>[2x]MSQQGLERRLLAGLQGLGLTINQAQRAVKHFGADALDRLEKDLFTLTEVEGIGFLTADKLWQARGGALDDPRRLTAAAVYALQLAGTQAGHSFLPRSRAEKGVVHYTRVTPGQARLAVETAVELGRLSEDDSPLFAAEAAATGEGRIYLPHVLRAEKKLASLIRTLLATPPADGAGNDDWAVPKKARKGLSEEQASVLDQLAGHRLVVLTGG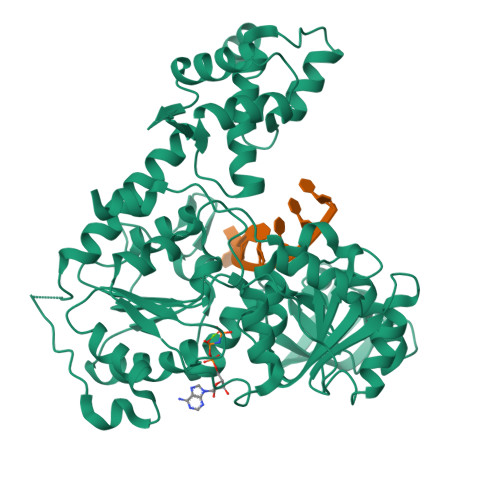PGTGKSTTTKAVADLAESLGLEVGLCAPTGKAARRLGEVTGRTASTVHRLLGYGPQGFRHNHLEPAPYDLLIVDEVSMMGDALMLSLLAAVPPGARVLLVGDTDQLPPVDAGLPLLALAQAAPTIKLTQVYRQAAKNPIIQAAHGLLHGEAPAWGDKRLNLTEIEPDGGARRVALMVRELGGPGAVQVLTPMRKGPLGMDHLNYHLQALFNPGEGGVRIAEGEARPGDTVVQTKNDYNNEIFNGTLGMVLKAEGARLTVDFDGNVVELTGAELFNLQLGYALTVHRAQGSEWGTVLGVLHEAHMPMLSRNLVYTALTRARDRFFSAGSASAWQIAAARQREARNTALLERIRAHLEHHHHHH>RPEWIWLALGTALMGLGTLYFLVKGMGVSDPDAKKFYAITTLVPAIAFTMYLSMLLGYGLTMVPFGGEQNPIYWARYADWLFTTPLLLLDLALLVDADQGTILALVGADGIMIGTGLVGALTKVYSYRFV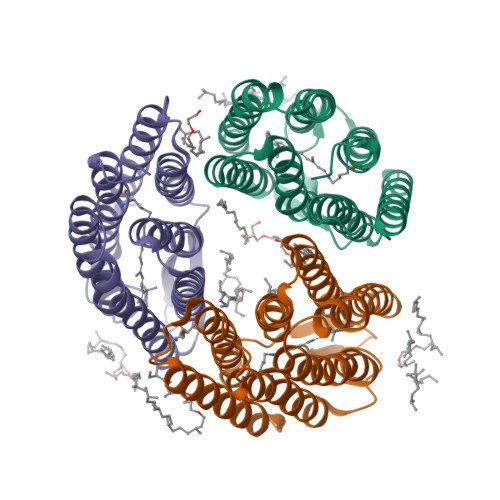WWAISTAAMLYILYVLFFGFTSKAESMRPEVASTFKVLRNVTVVLWSAYPVVWLIGSEGAGIVPLNIETLLFMVLDVSTKVGFGLILLRSRAIFG[3x]> DL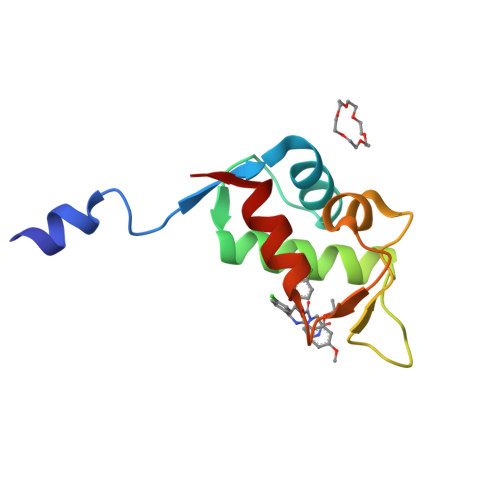ENLYFQGSQINQVRPKLPLLKILHAAGAQGEMFTVKEVMHYLGQYIMVKQLYDQQEQHMVYCGGDLLGELLGRQSFSVKDPSPLYDMLRKNLVT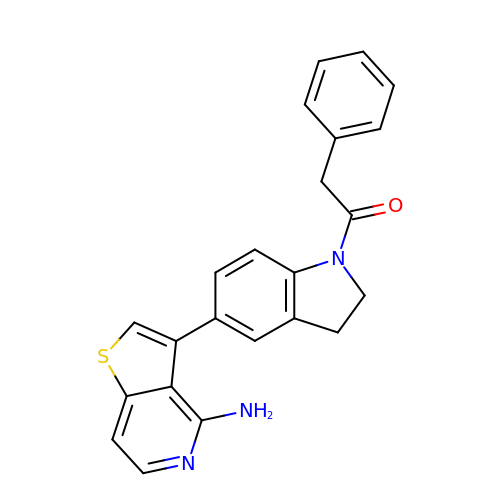1-[5-(4-aminothieno[3,2-c]pyridin-3-yl)-2,3-dihydro-1H-indol-1-yl]-2-phenylethanone | C23 H19 N3 O S | ZDMNFWRMUCKWCS-UHFFFAOYSA-N>[5x]MITVIAIAKDGSIVEPKLDEISFEDYRLIWIDCYDPKDEELYKLSKKIGISVSDLQIGLDEQEIPRVEEDEDFYLIIYKAPLFEEDITTTSLGIYIKNNLLLTIHSDKIKAIGRLHKLISTKKPRIVFERGIGFLLYHILNEITRSYSRILMNLEDELEELEDKLLAGYDREVMEKILGLRKTLVYF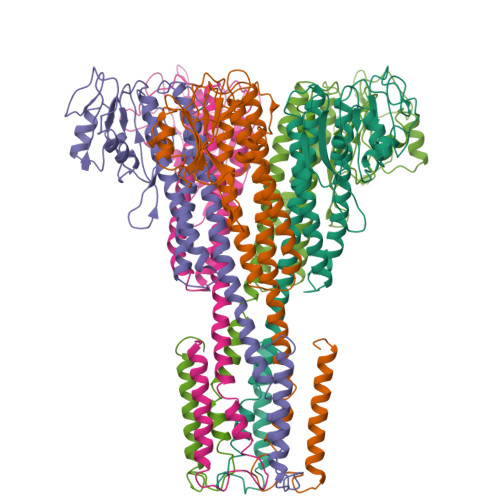HKSLIANRDVLVLLKRKYLPITTKEDRENFEDLYYDTLQLIDMSATYREVLTSMMDITLSLENIKMNQIMKILTMVTTIFAVPMWITGIYGMNFSYLPLANNPQGFWLVMALMVVIIMIFVYIFRRSGWI> MAPGEKIKAKIKKNLPVTGPQAPTIKELMRWYCLNTNTHGCRRIVVSRGRLRRLLWIGFTLTAVALILWQCALLVFSFYTVSVSIKVHFRKLDFPAVTICNINPYKYSTVRHLLADLEQETREALKSLYGFPESRKRREAESWNSVSEGKQPRFSHRIPLLIFDQDEKGKARDFFTGRKRKVGGSIIHKASNVMHIESKQVVGF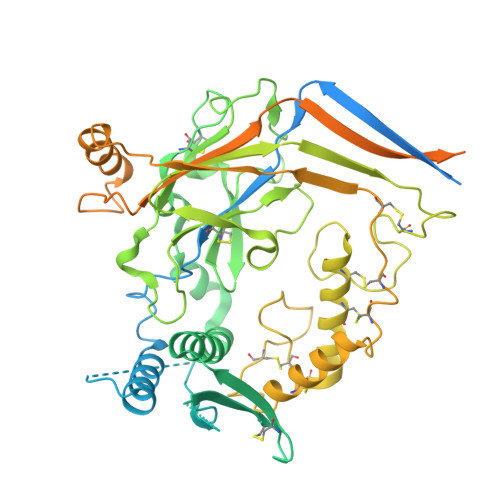QLCSNDTSDCATYTFSSGINAIQEWYKLHYMNIMAQVPLEKKINMSYSAEELLVTCFFDGVSCDARNFTLFHHPMHGNCYTFNNRENETILSTSMGGSEYGLQVILYINEEEYNPFLVSSTGAKVIIHRQDEYPFVEDVGTEIETAMVTSIGMHLTESFKLSEPYSQCTEDGSDVPIRNIYNAAYSLQICLHSCFQTKMVEKCGCAQYSQPLPPAANYCNYQQHPNWMYCYYQLHRAFVQEELGCQSVCKEACSFKEWTLTTSLAQWPSVVSEKWLLPVLTWDQGRQVNKKLNKTDLAKLLIFYKDLNQRSIMESPANSIEMLLSNFGGQLGLWMSCSVVCVIEIIEVFFIDFFSIIARRQWQKAKEWWAWKQAPPCPEAPRSPQGQDNPALDIDDDLPTFNSALHLPPALGTQVPGTPPPKYNTLRLERAFSNQLTDTQMLDEL>[4x]MKGKMAIVISTLNNPWFVVLAETAKQRAEQLGYEATIFDSQNDTAKESAHFDAIIAAGYDAIIFNPTDADGSIANVKRAKEAGIPVFCVDRGINARGLAVAQIYSDTSTQFPKLMARLAVEWADQYLRGGLEHHHHHH

Periplasmic binding proteins (PBPs) are a class of proteins that participate in the cellular transport of various ligands. The structurally symmetric bilobal architecture of their fold has long been thought to originate from a duplication and fusion event of an individual lobe. Here, the crystal structures of two permuted halves of a modern ribose-binding protein (RBP) from Thermotoga maritima are reported.

RBP-CPN was designed to consist only of the βA–Eα1–4 elements, which are directly linked to α9. In the concentration range 0.5–5 mg ml−1, the determined molecular weight (MW) of RBP-CPN is approximately 27.5 kDa. This corresponds to a dimeric conformation, as it is about double the expected monomeric MW of 14.9 kDa. The crystal structure of RBP-CPN was solved in the monoclinic space group P21 at 1.79 Å resolution. The asymmetric unit is composed of four chains, of which two pairs form a dimer via a segment swap. Unlike the interface of the two lobes in native PBPs, the dimer is located on the edge of the two central β-sheets. In contrast to the rest of the central β-sheet, the two βE strands form an antiparallel stretch of the extended β-sheet. The novel antiparallel stretch of the dimer-swapped β-sheets has not been observed before in proteins with the type I PBP-like fold, and the existence of this swap highlights the flexibility of this structural element.>ETGHHHHHHSADEPMDFKINTDEIMTSLKSVNGQIESLISPDGSRKNPARNCRDLKFCHPELKSGEYWVDPNQGCKLDAIKVFCNMETGETCISANPLNVPRKHWWTDSSAEKK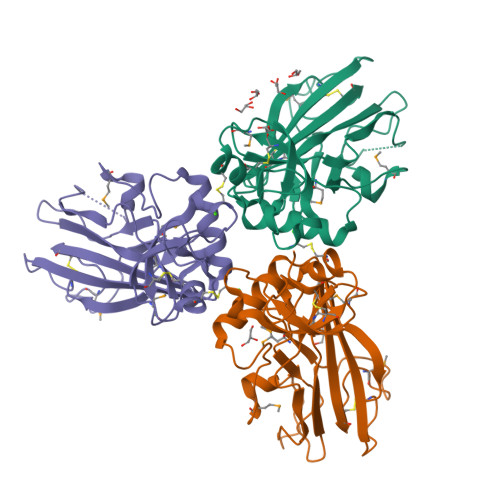HVWFGESMDGGFQFSYGNPELPEDVLDVQLAFLRLLSSRASQQITYHCKNSIAYMDQASGNVKKALKLMGSNEGEFKAEGNSKFTYTVLEDGCTKHTGEWSKTVFEYRTRKAVRLPIVDIAPYDIGGPDQEFGVDVGPVCFL[3x]The first enzyme in the pathway, peptide O-xylosyltransferase (XT, EC 2.4.2.26), catalyzes the transfer of xylose from uridine diphosphate (UDP)-α-D-xylose onto serine and thus determines the site(s) of GAG attachment on the core protein. XT1 and XT2 are type II transmembrane proteins consisting of a short amino-terminal region facing the cytosol, a single transmembrane helix, a stem region required for Golgi localization (Schön et al., 2006), a catalytic GT-A domain (Lairson et al., 2008, Müller et al., 2006), and a unique C-terminal domain of unknown function, termed “Xylo_C” in the Pfam database (Finn et al., 2008). XT1 has a two-lobed structure, with one lobe comprising the catalytic GT-A domain and the other comprising the Xylo_C domain. To better understand the initial step of GAG biosynthesis, we have determined crystal structures of human XT1 complexed with UDP-xylose and various PG-derived acceptor peptides.

To visualize how the different amino acid substitutions are accommodated in the peptide binding cleft, we selected five variants of the bikunin-derived peptide for structure analysis (peptides 3–7). The +2 position exhibited an unexpected preference for the β-branched amino acid valine (and, to a lesser extent, threonine). The substitution of glycine by valine at position +2 (peptide 6) results in a 72° rotation of the 217-218 peptide bond, which allows K461 to form a new hydrogen bond with the backbone carbonyl of the peptide at the −2 position. This induces a kink in the peptide, pulling the glutamic acid side chain at position −2 out of the binding site and replacing it with that of the glutamic acid at position −3. To accommodate this rearrangement the 449–466 loop moves slightly, widening the peptide binding cleft by ∼3 Å.

> APLVHHHHHHALDENLYFQGALADVSRPPHARKTGGSSPETKYDQPPKCDISGKEAISALSRAKSKHCRQEIGETYCRHKLGLLMPEKVTRFCPLEGKANKNVQWDEDSVEYMPANPVRIAFVLVVHGRASRQLQRMFKAIYHKDHFYYIHVDKRSNYLHRQVLQVSRQYSNVRVTPWRMATIWGGASLLSTYLQSMRDLLEMTDWPWDFFINLSAADYPIRTNDQLVAFLSRYRDMNFLKSHGRDNARFIRKQGLDRLFLECDAHMWRLGDRRIPEGIAVDGGSDWFLLNRRFVEYVTFSTDDLVTKMKQFYSYTLLPAESFFHTVLENSPHCDTMVDNNLRITNWNRKLGCKCQYKHIVDWCGCSPNDFKPQDFHRFQQTARPTFFARKFEAVVNQEIIGQLDYYLYGNYPAGTPGLRSYWENVYDEPDGIHSLSDVTLTLYHSFARLGLRRAETSLHTDGENSCRYYPMGHPASVHLYFLADRFQGFLIKHHATNLAVSKLETLETWVMPKKVFKIASPPSDFGRLQFSEVGTDWDAKERLFRNFGGLLGPMDEPVGMQKWGKGPNVTVTVIWVDPVNVIAATYDILIESTAEFTHYKPPLNLPLRPGVWTVKILHHWVPVAETKFLVAPLTFSNRQPIKPEEALKLHNGPLRNAYMEQSFQSLNPVLSLPINPAQVEQARRNAASTGTALEGWLDSLVGGMWTAMDICATGPTACPVMQTCSQTAWSSFSPDPKSELGAVKPDGRLR;> QEEEGSGVGQGG> GSNNVLPTWSLDSNGEMRSRLSLSEVLDSGDLMKFAVDKTGCQFLEKAVKGSLTSYQKFQLFEQVIGRKDDFLKLSTNIFGNYLVQSVIGISLATNDDGYTKRQEKLKNFISSQMTDMCLDKFACRVIQSSLQNMDLSLACKLVQALPRDARL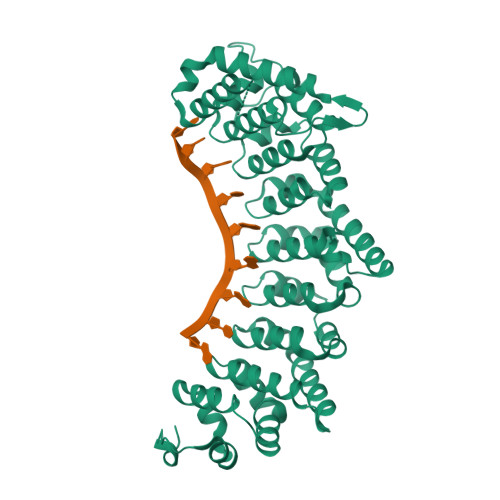IAICVDQNANHVIQKVVAVIPLKNWEFIVDFVATPEHLRQICSDKYGCRVVQTIIEKLTADSMNVDLTSAAQNLRERALQRLMTSVTNRCQELATNEYANYIIQHIVSNDDLAVYRECIIEKCLMRNLLSLSQEKFASHVVEKAFLHAPLELLAEMMDEIFDGYIPHPDTGKDALDIMMFHQFGNYVVQCMLTICCDAVSGRRQTKEGGYDHAISFQDWLKKLHSRVTKERHRLSRFSSGKKMIETLANLRSTHPIYELQSSGHDSFKTDYFSTASEHDGPELEKNGIEEGSLMLEPRSNKSSVSVKFSSSGSHGDD>AEKPKLHYFNARGRMESTRWLLAAAGVEFEEKFIKSAEDLDKLRNDGYLMFQQVPMVEIDGMKLVQTRAILNYIASKYNLYGKDIKERALIDMYIEGIADLGEMILLLPVXPPEEKDAKLALIKEKIKNRYFPAFEKVLKSHGQDYLVGNKLSRADIHLVELLYYVEELDSSLISSFPLLKALKTRISNLPTVKKFLQPGSPRKPPMDEKSLEEARKIFRF[4x]

Glutathione S-transferases (GST) are involved in the metabolism of PEITC by catalyzing its conjugation with glutathione (GSH). As phase II detoxification enzymes, cytosolic GSTs exist and function as stable homo- or heterodimers. The dimer is required to maintain the functional conformations at the GSH-binding site and xenobiotic substrate-binding site in each subunit. Here, we report the crystal structures of hGSTP1 and hGSTA1 in complex with GS-PEITC (hGSTP1:GS-PEITC and hGSTA1:GS-PEITC, respectively).

We determined the crystal structures of the hGSTA1:GS-PEITC and hGSTP1:GS-PEITC complexes at 1.93- and 1.95-Å resolution, respectively. The structures show that the orientation of the phenethyl moiety of the conjugate was significantly different in the two GST enzymes. In the hGSTA1:GS-PEITC structure, the phenethyl moiety of GS-PEITC docks into a hydrophobic pocket formed by the side chains of Leu107, Leu108, Val111, Met208, Leu213, Phe222, Phe10 and Phe220. The hGSTA1 contains a single cysteine residue, Cys112. The hGSTA1:GS-PEITC structure reveals that the side chain of Cys112 was covalently modified by PEITC. Like the sulfhydryl group of GSH, the sulfhydryl group of Cys112 acts as a nucleophile and attacks the isothiocynate central C atom of PEITC and forms an irreversible adduct with hGSTA1 (hGSTA1Cys112-PEITC). In the hGSTA1 dimer, the Cys112 pair is located near the entrance of the solvent channel at the subunit interface. One can imagine that the covalent modification of both Cys112 side chains with PEITC must have significant impact on the dynamics of the interface, the openness of the solvent channel, the binding of GSH and substrate, and the release of the product. Indeed, the formation of Cys112-PEITC in hGSTA1 did alter the catalytic activity significantly, leading to more than two orders of magnitude inhibition in vitro.>GSHMNGPIIMTREERMKIVHEIKERILDKYGDDVKAIGVYGSLGRQTDGPYSDIDMMCVMSTEEAEFSHEWTTGEWKVEVNFDSEEILLDYASQVESDWPLTHGQFFSILPIYDSGGYLEKVYQTAKSVEAQKFHDAICALIVEELFEYAGKWRNIRVQGPTTFLPSLTVQVAMAGAMLIGLHHRICYTTSASVLTEAVKQSDLPSGYDHLCQFVMSGQLSD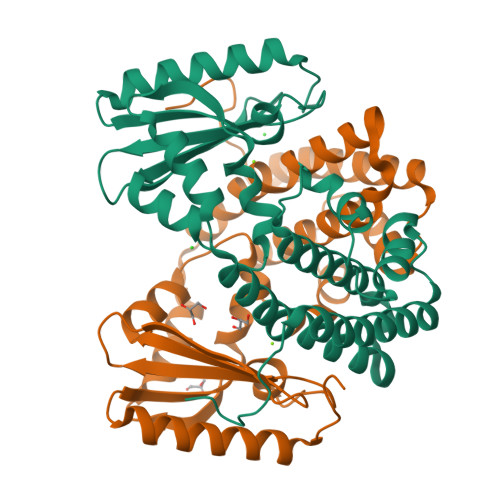SEKLLESLENFWNGIQEWTERHGYIVDVSKRIPF[2x]>[3x]MIIPALNLIGGTVVRVVRLHQGDYARLRDYGNDPLPRLQDYAAQGAGVLHLVDLTGAKDPAKRQIPLIKTLVAGVNVPVQVGGGVRTEEDVAALLKAGVARVVIASTAVKSPDVVKGWFERF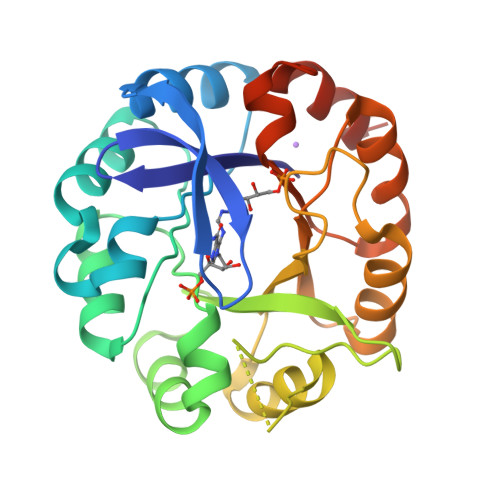GAQALVLALDVRIDEHGTKQVAVSGWQENSGVSLEQLVETYLPVGLKHVLCTDISRDGTLAGSNVSLYEEVCARYPQIAFQSSGGIGDIDDIAALRGTGVRGVIVGRALLEGKFTVKEAIQCWQNVKGHHHHHH> GSHMGEKRSIAIDSYQEDPSVVVSNFFKGVRVPKDTEFQLYKKRKQDQFV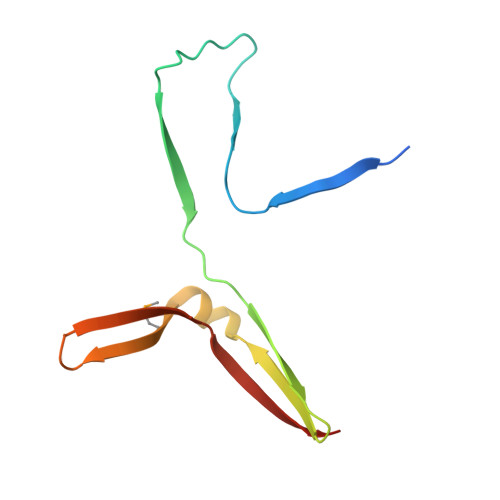LHGENERLEYDGETDELTTKTNQYMVGLYDKQSGKINLYRAPVVTSKIVSKF>QTSPMTPDITGKPFVAADAS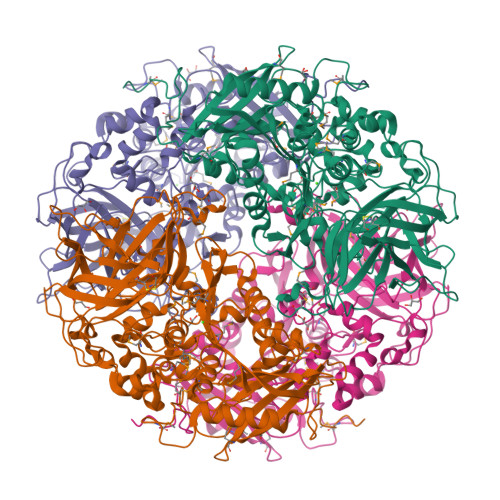NDYIKREVMIPMRDGVKLHTVIVLPKGAKNAPIVLTRTPYDASGRTERLASPHMKDLLSAGDDVFVEGGYIRVFQDVRGKYGSEGDYVMTRPLRGPLNPSEVDHATDAWDTIDWLVKNVSESNGKVGMIGSSYEGFTVVMALTNPHPALKVAVPESPMIDGWMGDDWFNYGAFRQVNFDYFTGQLSKRGKGAGIARQGHDDYSNFLQAGSAGDFAKAAGLEQLPWWHKLTEHAAYDAFWQEQALDKVMARTPLKVPTMWLQGLWDQEDMWGAIHSYAAMEPRDKRNTLNYLVMGPWRHSQVNYDGSALGALNFEGDTARQFRHDVLRPFFDQYLVDGAPKADTPPVFIYNTGENHWDRLKAWPRSCDKGCAATSKPLYLQAGGKLSFQPPVAGQAGFEEYVSDPAKPVPFVPRPVDFADRAMWTTWLVHDQRFVDGRPDVLTFVTEPLTEPLQIAGAPDVHLQASTSGSDSDWVVKLIDVYPEEMASNPKMGGYELPVSLAIFRGRYRESFSTPKPLTSNQPLAFQFGLPTANHTFQPGHRVMVQVQSSLFPLYDRNPQTYVPNIFFAKPGDYQKATQRVYVSPEQPSYISLPVR[4x]> MAAPQFHRPSTITADNVRALGMRGLVLATNNAQFIMDNSYPHPHGTQGAVREFLR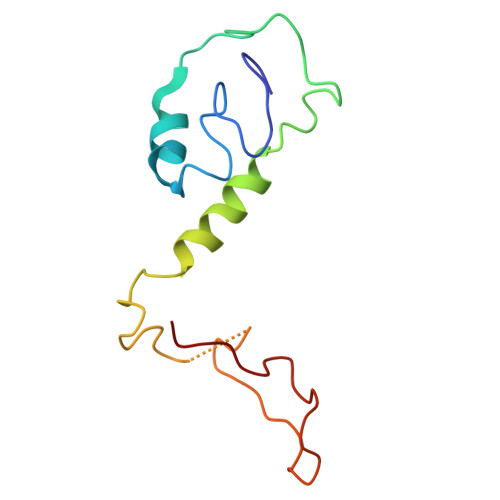GQAAALTDLGVTHANNTFAPQPMFAGDAAAEWLRPSFGLKRTYSPFVVRDPKTPSTP>[6x]MSLPDGFYIRRMEEGDLEQVTETLKVLTTVGTITPESFCKLIKYWNEATVWNDNEDKKIMQYNPMVIVDKRTETVAATGNIII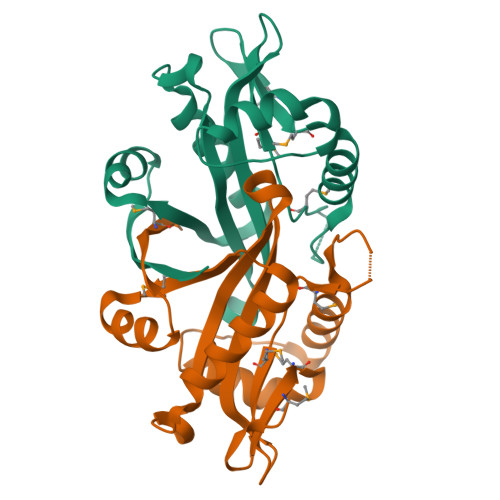ERKIIHELGLCGHIEDIAVNSKYQGQGLGKLLIDQLVTIGFDYGCYKIILDCDEKNVKFYEKCGFSNAGVEMQIRK> MRGMLPLFEPKGRVLLVDGHHLAYRTFHALKGLTTSRGEPVQAVYGFAKSLLKALKEDGDAVIVVFDAKAPSFRHEAYGGYKAGRAPTPEDFPRQLALIKELVDLLGLARLEVPGYEADDVLASLAKKAEKEGYEVRILTADKDLYQLLSDRIHVLHPEGYLITPAWLWEKYGLRPDQWADYRALTGDESDNLPGVKGIGEKTARKLLEEWGSLEALLKNLDRLKPAIREKILAHMDDLKLSWDLAKVRTDLPLEVDFAKRREPDRERLRAFLERLEFGSLLHEFGLLESPKALEEAPWPPPEGAFVGFVLSRKEPMWADLLALAAARGGRVHRAPEPYKALRDLKEARGLLAKDLSVLALREGLGLPPGDDPMLLAYLLDPSNTTPEGVARRYGGEWTEEAGERAALSERLFANLWGRLEGEERLLWLYREVERPLSAVLAHMEATGVRLDVAYLRALSLEVAEEIARLEAEVFRLAGHPFNLNSRDQLERVLFDELGLPAIGKTEKTGKRSTSAAVLEALREAHPIVEKILQYRELTKLKSTYIDPLPDLIHPRTGRLHTRFNQTATATGRLSSSDPNLQNIPVRTPLGQRIRRAFIAEEGWLLVALDYSQIELRVLAHLSGDENLIRVFQEGRDIHTETASWMFGVPREAVDPLMRRAAKTINFGVLYGMSAHRLSQELAIPYEEAQAFIERYFQSFPKVRAWIEKTLEEGRRRGYVETLFGRRRYVPDLEARVKSVREAAERMAFNMPVQGTAADLMKLAMVKLFPRL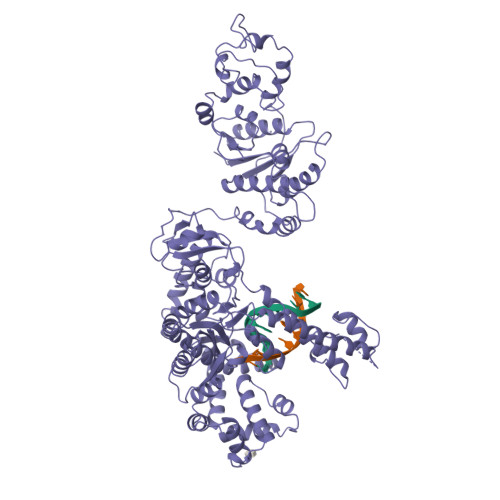EEMGARMLLQVHDELVLEAPKERAEAVARLAKEVMEGVYPLAVPLEVEVGIGEDWLSAKE(1S)-2-methyl-1-(2-methyl-1,2,4-triazol-3-yl)propan-1-amine 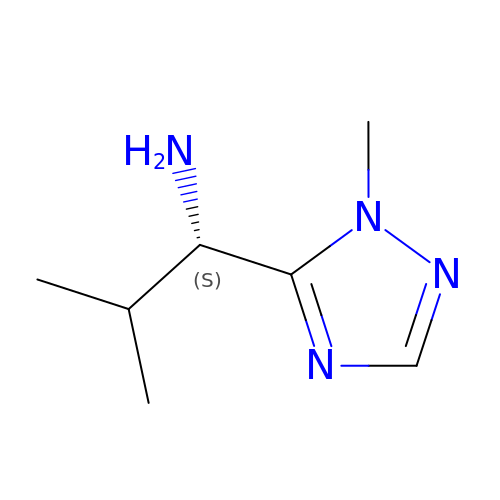| C7 H14 N4 | LUTYSHHATVYMSC-LURJTMIESA-N> SSLDDKPQFPGASAEFIDKLEFIQPNVISGIPIYRVMDRQGQIINPSEDPHLPKEKVLKLYKSMTLLNTMDRILYESQRQGRISFYMTNYGEEGTH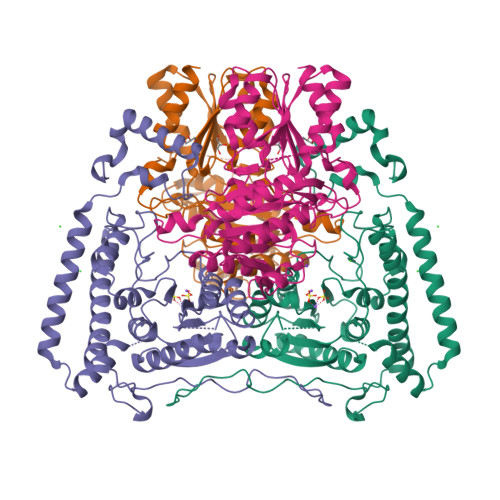VGSAAALDNTDLVFGQYREAGVLMYRDYPLELFMAQCYGNISDLGKGRQMPVHYGCKERHFVTISSPLATQIPQAVGAAYAAKRANANRVVICYFGEGAASEGDAHAGFNFAATLECPIIFFCRNNGYAISTPTSEQYRGDGIAARGPGYGIMSIRVDGNDVFAVYNATKEARRRAVAENQPFLIEAMTYRIGHASTSDDSSAYRSVDEVNYWDKQDHPISRLRHYLLSQGWWDEEQEKAWRKQSRRKVMEAFEQAERKPKPNPNLLFSDVYQEMPAQLRKQQESLARHLQTYGEHYPLDHFDK;> VAHFTFQPDPEPREYGQTQKMNLFQSVTSALDNSLAKDPTAVIFGEDVAFGGVFRCTVGLRDKYGKDRVFNTPLCEQGIVGFGIGIAVTGATAIAEIQFADYIFPAFDQIVNEAAKYRYRSGDLFNCGSLTIRSPWGCVGHGALYHSQSPEAFFAHCPGIKVVIPRSPFQAKGLLLSCIEDKNPCIFFEPKILYRAAAEEVPIEPYNIPLSQAEVIQEGSDVTLVAWGTQVHVIREVASMAKEKLGVSCEVIDLRTIIPWDVDTICKSVIKTGRLLISHEAPLTGGFASEISSTVQEECFLNLEAPISRVCGYDTPFPHIFEPFYIPDKWKCYDALRKMINY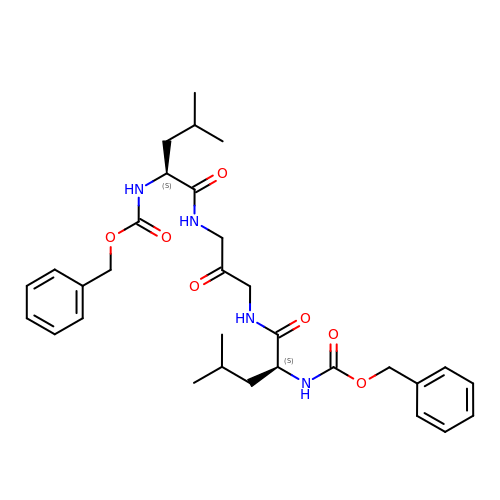1,3-BIS[[N-[(PHENYLMETHOXY)CARBONYL]-L-LEUCYL]AMINO]-2-PROPANONE | C31 H42 N4 O7 | APGQPPIXNOCMOK-SVBPBHIXSA-N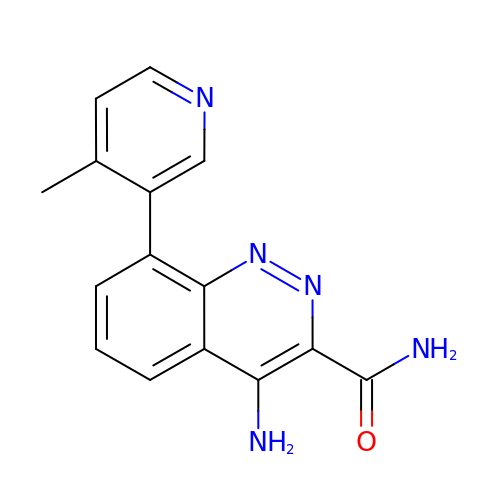4-amino-8-(4-methylpyridin-3-yl)cinnoline-3-carboxamide | C15 H13 N5 O | YHEHDRMGAHEUOQ-UHFFFAOYSA-N> FSQHARTSGRVAVEEVDEEGKFVRLRNKSNEDQSMGNWQIKRQNGDDPLLTYRFPPKFTLKAGQVVTIWAAGAGATHSPPTDLVWKAQNTWGCGNSLRTALIN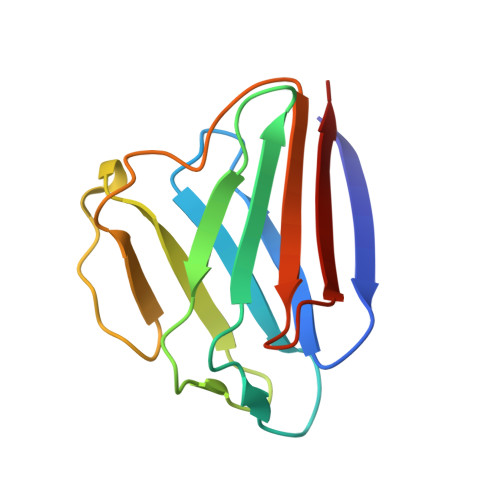STGEEVAMRKLVR>[2x]TNILAGAAVIKVLEAWGVDHLYGIPGGSINSIMDALSAERDRIHYIQVRHEEVGAMAAAADAKLTGKIGVCFGSAGPGGTHLMNGLYDAREDHVPVLALIGQFGTTGMNMDTFQEMNENPIYADVADYNVTAVNAATLPHVIDEAIRRAYAHQGVAVVQIPVDLPWQQISAEDWYASANNYQTPLLPEPDVQAVTRLTQTLLAAERPLIYYGIGARKAGKELEQLSKTLKIPLMSTYPAKGIVADRYPAYLGSANRVAQKPANEALAQADVVLFVGNNYPFAEVSKAFKNTRYFLQIDIDPAKLGKRHKTDIAVLADAQKTLAAILAQVSERESTPWWQANLAN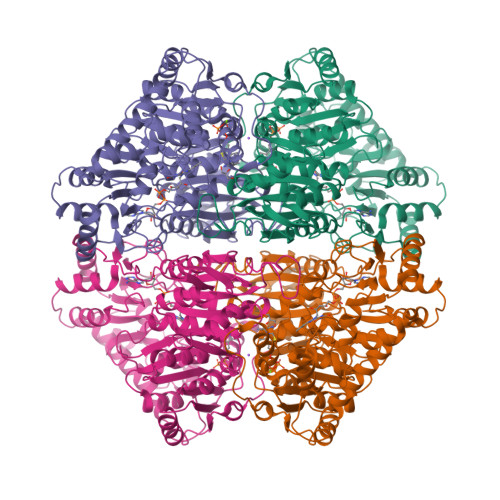VKNWRAYLASLEDKQEGPLQAYQVLRAVNKIAEPDAIYSIDVGDINLNANRHLKLTPSNRHITSNLFATMGVGIPGAIAAKLNYPERQVFNLAGDGGASMTMQDLVTQVQYHLPVINVVFTNCQYGFIKDEQEDTNQNDFIGVEFNDIDFSKIADGVHMQAFRVNKIEQLPDVFEQAKAIAQHEPVLIDAVITGDRPLPAEKLRLDSAMSSAADIEAFKQRYEAQDLQPLSTYLKQFGLDD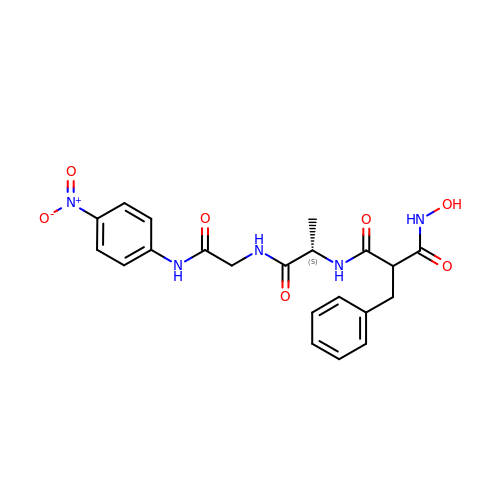HONH-BENZYLMALONYL-L-ALANYLGLYCINE-P-NITROANILIDE | C21 H23 N5 O7 | TZWQPWGUQCSKDW-GUYCJALGSA-N> GVTFDDGAYTGIREINFEYNSETAIGGLRVTYDLNGMPFVAEDHKSFITGFKPVKISLEF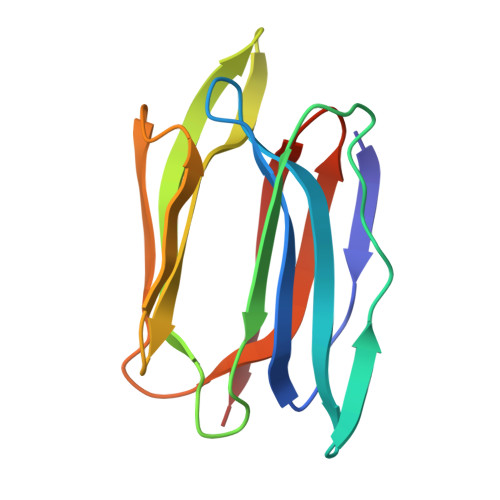PSEYIVEVSGYVGKVEGYTVIRSLTFKTNKQTYGPYGVTNGTPFSLPIENGLIVGFKGSIGYWLDYFSIYLSL>[2x]SMSTNGDDHQVKDSLEQLRCHFTWELSIDDDEMPDLENRVLDQIEFLDTKYSVGIHNLLAYVKHLKGQNEEALKSLKEAENLMQEEHDNQANVRSLVTWGNFAWMYYHMGRLAEAQTYLDKVENICKKLSNPFRYRMECPEIDCEEGWALLKCGGKNYERAKACFEKVLEVDPENPESSAGYAISAYRLDGFKLATKNHKPFSLLPLRQAVRLNPDNGYIKVLLALKLQDEGQEAEGEKYIEEAL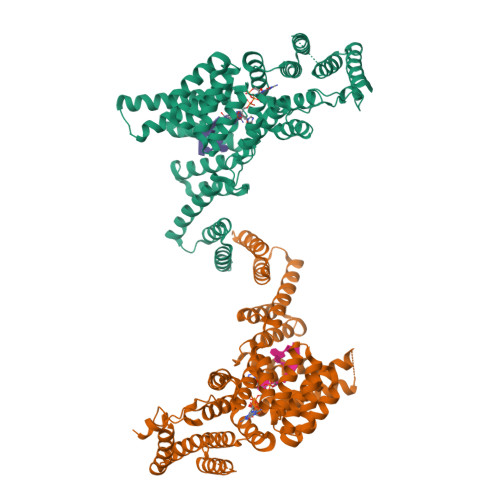ANMSSQTYVFRYAAKFYRRKGSVDKALELLKKALQETPTSVLLHHQIGLCYKAQMIQIKEATKGQPRGQNREKLDKMIRSAIFHFESAVEKKPTFEVAHLDLARMYIEAGNHRKAEENFQKLLCMKPVVEETMQDIHFHYGRFQEFQKKSDVNAIIHYLKAIKIEQASLTRDKSINSLKKLVLRKLRRKALDLESLSLLGFVYKLEGNMNEALEYYERALRLAADFENSVRQGP> GTEETAKVVPMAVITPAINQLTDQEKAEGWALLFDGKTTKGWRGAHKDAFPDHGWMVKDGELIVQKSDGSESTNGGDIVTEGEYSAFEFSVDFKITEGANSGIKYFVTEQEKQKGSAYGLEFQLLDDAKHPDAKLYTTFPGSRTLGSLYD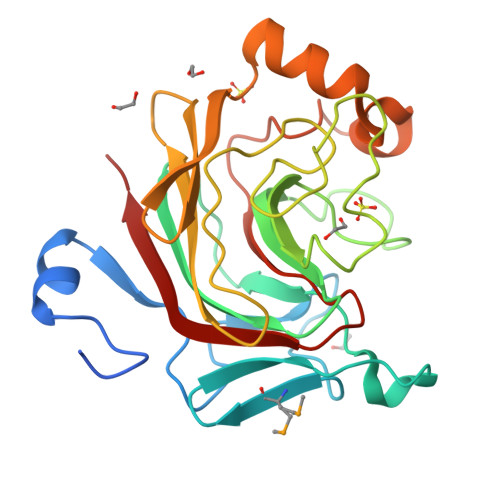LKKSENIHFNGVGEWNTAVVKVFPNNHVEHWLNGVKVLEYERGSKEFRDLVKGSKYADPSYNAGGAFGEAPKGHILLQDHGDEVAFRNIKVKELK> MAVKIKIEHLTKIFGKRIKTALTMVEKGEPKNEILKKTGATVGVYDTNFEINEGEIFV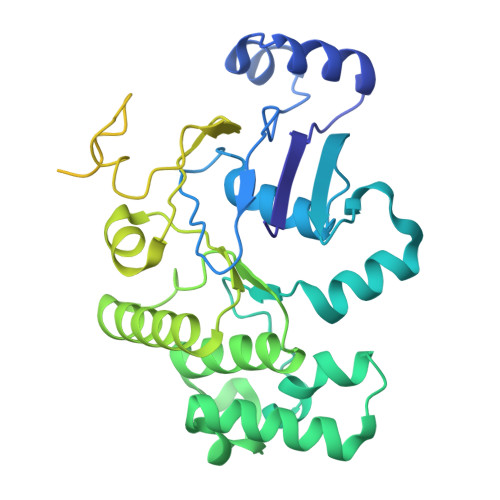IMGLSGSGKSTLLRLLNRLIEPTSGKIFIDNQDVATLNKEDLLQVRRKTMSMVFQNFGLFPHRTILENTEYGLEVQNVPKEERRKRAEKALDNANLLDFKDQYPKQLSGGMQQRVGLARALANDPEILLMDEAFSALDPLIRREMQDELLELQAKFQKTIIFVSHDLNEALRIGDRIAIMKDGKIMQIGTGEEILTNPANDYVKTFVEDVDRAKVITAENIMIPALTTNIDVDGPSVALKKMKTEEVSSLMAVDKKRQFRGVVTSEQAIAARKNNQPLKDVMTTDVGTVSKEMLVRDILPIIYDAPTPLAVVDDNGFLKGVLIRGSVLEALADIPDEDEVEEIEKEEENK>[4x]MTARAVRGTKDLFGK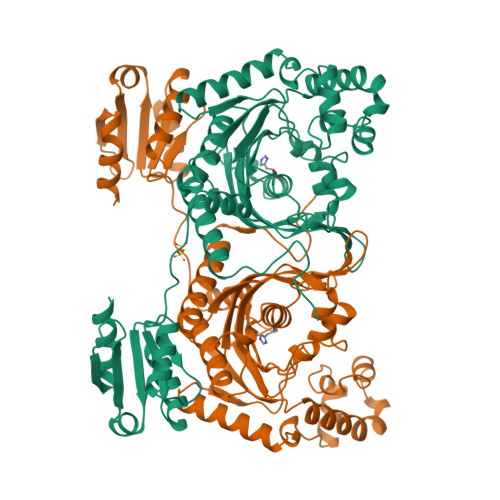ELRMHQRIVATARKVLEAAGALELVTPIFEETQVFEKGVGAATDIVRKEMFTFQDRGGRSLTLRPEGTAAMVRAYLEHGMKVWPQPVRLWMAGPMFRAERPQKGRYRQFHQVNYEALGSENPILDAEAVVLLYECLKELGLRRLKVKLSSVGDPEDRARYNAYLREVLSPHREALSEDSKERLEENPMRILDSKSERDQALLKELGVRPMLDFLGEEARAHLKEVERHLERLSVPYELEPALVRGLDYYVRTAFEVHHEEIGAQSALGGGGRYDGLSELLGGPRVPGVGFAFGVERVALALEAEGFGLPEEKGPDLYLIPLTEEAVAEAFYLAEALRPRLRAEYALAPRKPAKGLEEALKRGAAFAGFLGEDELRAGEVTLKRLATGEQVRLSREEVPGYLLQALG> AESTLGAAAAQSGRYFGTAIASGRLSDSTYTSIAGREFNMVTAENEMKIDATEPQRGQFNFSSADRVYNWAVQNGKQVRGHTLAWHSQQPGWMQSLSGSALRQAMIDHINGVMAHYKGKIVQWDVVNEAFADGSSGARRDSNLQRSGNDWIEVAFRTARAADPSAKLCYNDYNVENWTWAKTQAMYNMVRDFKQRGVPIDCVGFQSHFNSGSPYNSNFRTTLQNFAALGVDVAITELDIQGAPASTYANVTNDCLAVSRCLGITVWGVRDSDSWRSEQTPLLFNNDGSKKAAYTAVLDAL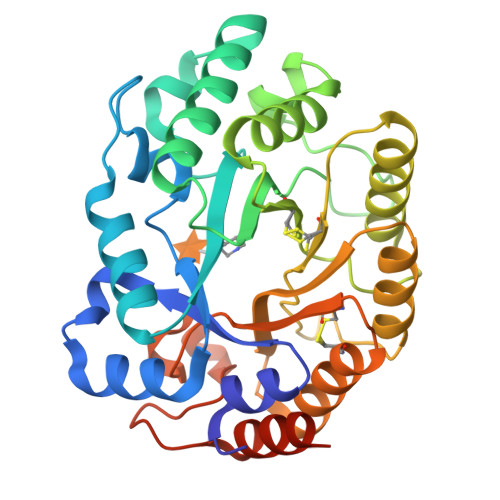NGGDSSEPPADGG>[4x]GKNGKGEVIIPKEKFWKISTPPEAYWNREQEKLNRQYNPILSMLTNQTGEAGRLSNISHLNYCEPDLRVTSVVTGFNNLPDRFKDFLLYLRCRNYSLLIDQPDKCAKKPFLLLAIKSLTPHFARRQAIRESWGQESNAGNQTVVRVFLLGQTPPEDNHPDLSDMLKFESEKHQDILMWNYRDTFFNLSLKEVLFLRWVSTSCPDTEFVFKGDDDVFVNTHHILNYLNSLSKTKAKDLFIGDVIHNAGPHRDKKLKYYIPEVVYSGLYPPYAGGGGFLYSGHLALRLYHITDQVHLYPIDDVYTGMCLQKLGLVPEKHKGFRTFDIEEKNKNNICSYVDLMLVHSRKPQEMIDIWSQLQSAHLKC

The majority of mammalian poly-LacNAc is synthesized by the alternating iterative action of β1,3-N-acetylglucosaminyltransferase 2 (B3GNT2) and β1,4-galactosyltransferases. B3GNT2 is in the largest mammalian glycosyltransferase family, GT31, but little is known about the structure, substrate recognition, or catalysis by family members. Here we report the structures of human B3GNT2 in complex with UDP:Mg2+ and in complex with both UDP:Mg2+ and a glycan acceptor, lacto-N-neotetraose. The B3GNT2 structure conserves the GT-A fold and the DxD motif that coordinates a Mg2+ ion for binding the UDP-GlcNAc sugar donor.

Unlabeled B3GNT2:UDP:Mg2+ crystallized in a different space group and was solved at 2.04 Å resolution. Despite differences in crystal packing, the SeMet-B3GNT2:UDP:Mg2+ and B3GNT2:UDP:Mg2+ structures are essentially the same, with the latter revealing the same dimeric complex formed by crystallographic symmetry. In the acceptor-free B3GNT2:UDP:Mg2+ and SeMet-B3GNT2:UDP:Mg2+ complexes, the Asp333 and Gly-Loop305:307 are only observed in the inactive conformation despite the fact that the latter structure was solved in a crystal form that is isomorphous to the B3GNT2:UDP:Mg2+:LNnT complex. This suggests acceptor binding contributes to the stabilization of the active state conformation of the enzyme.> HMSNFTGLKVLVMDENGVSRMVTKGLLVHLGCEVTTVSSNEECLRVVSHEHKVVFMDVCMPGVENYQIALRIHEKFTKQRHQRPLLVA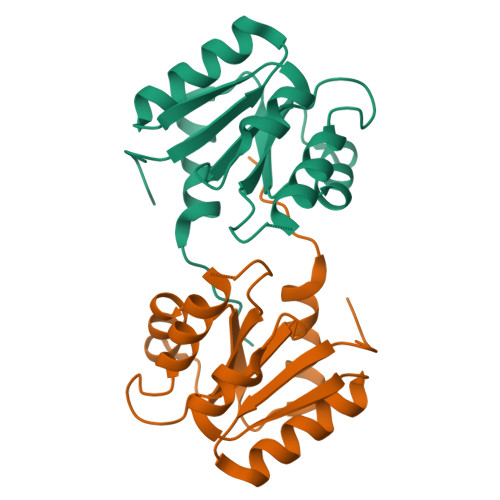LSGNTDKSTKEKCMSFGLDGVLLKPVSLDNIRDVLSDLLEPRVLYEGM>[2x]ASAWPEEKNYHQPAILNSSALRQIAEGTSISEMWQNDLQP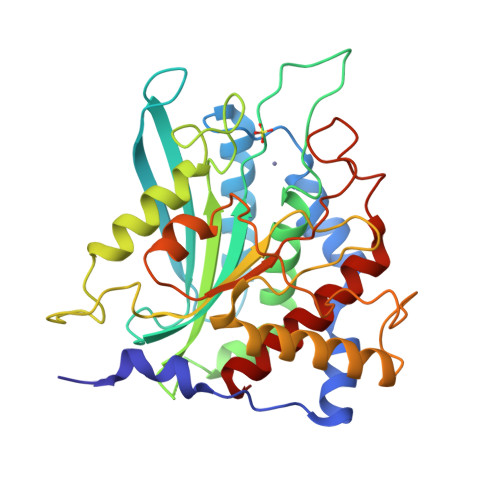LLIERYPGSPGSYAARQHIMQRIQRLQADWVLEIDTFLSQTPYGYRSFSNIISTLNPTAKRHLVLACHYDSKYFSHWNNRVFVGATDSAVPCAMMLELARALDKKLLSLKTVSDSKPDLSLQLIFFDGQEAFLHWSPQDSLYGSRHLAAKMASTPHPPGARGTSQLHGMDLLVLLDLIGAPNPTFPNFFPNSARWFERLQAIEHELHELGLLKDHSLEGRYFQNYSYGGVIQDDHIPFLRRGVPVLHLIPSPFPEVWHTMDDNEENLDESTIDNLNKILQVFVLEYLHL> ARTEPDEQDAVYD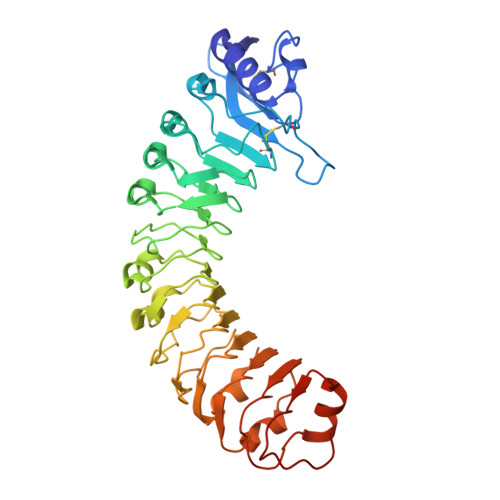IMRATGNDWAAAIPDVCRGRWHGIECMPDQDNVYHVVSLSFGALSDDTAFPTCDPQRSYVSESLTRLKHLKALFFYRCLGRAPQRIPAFLGRLGSSLQTLVLRENGFLGPIPDELGNLTNLKVLDLHKNHLNGSIPLSFNRFSGLRSLDLSGNRLTGSIPGFVLPALSVLDLNQNLLTGPVPPTLTSCGSLIKIDLSRNRVTGPIPESQNRLNQLVLLDLSYNRLSGPFPSSLQGLNSLQALMLKGNNKFSTTIPENAFKGLKNLMILVLSNTNIQGSIPKSLTRLNSLRVLHLEGNNLTGEIPLEFRDVKHLSELRLNDNSLTGPVPFERDTVWRMRRKLRLYNNAGLCVNRDSDAAAAF N-[2-(4-hydroxyphenyl)ethyl]pyridine-2-carboxamide | C14 H14 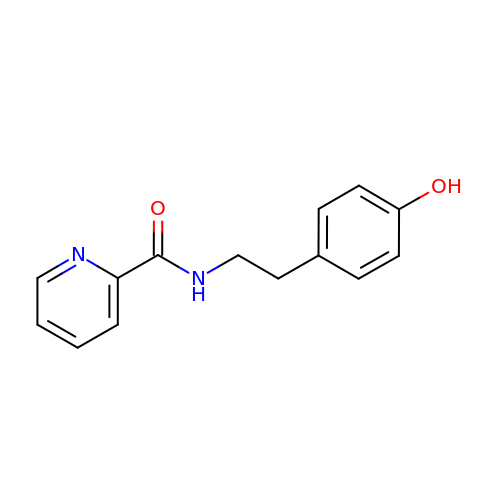N2 O2 | YXENGKAXLJYJOP-UHFFFAOYSA-N> MQNSQDFSITELSLPKGGGAITGMGEALTPTGPDGMAALSLPLPISAGRGYAPAFTLNYNSGAGNSPFGLGWDCNVMTIRRRTHFGVPHYDETDTFLGPEGEVLVVADQPRDESTLQGINLGATFTVTGYRSRLESHFSRLEYWQPKTTGKTDFWLIYSPDGQVHLLGKSPQARISNPSQTTQTAQWLLEASVSSRGEQIYYQYRAEDDTGCEADEITHHLQATAQRYLHIVYYGNRTASETLPGLDGSAPSQADWLFYLVFDYGERSNNLKTPPAFSTTGSWLCRQDRFSRYEYGFEIRTRRLCRQVLMYHHLQALDSKITEHNGPTLVSRLILNYDESAIASTLVFVRRVGHEQDGNVVTLPPLELAYQDFSPRHHAHWQPMDVLANFNAIQRWQLVDLKGEGLPGLLYQDKGAWWYRSAQRLGEIGSDAVTWEKMQPLSVIPSLQSNASLVDINGDGQLDWVITGPGLRGYHSQRPDGSWTRFTPLNALPVEYTHPRAQLADLMGAGLSDLVLIGPKSVRLYANTRDGFAKGKDVVQSGEITLPVPGADPRKLVAFSDVLGSGQAHLVEVSATKVTCWPNLGRGRFGQPITLPGFSQPATEFNPAQVYLADLDGSGPTDLIYVHTNRLDIFLNKSGNGFAEPVTLRFPEGLRFDHTCQLQMADVQGLGVASLILSVPHMSPHHWRCDLTNMKPWLLNEMNNNMGVHHTLRYRSSSQFWLDEKAAALTTGQTPVCYLPFPIHTLWQTETEDEISGNKLVTTLRYARGAWDGREREFRGFGYVEQTDSHQLAQGNAPERTPPALTKNWYATGLPVIDNALSTEYWRDDQAFAGFSPRFTTWQDNKDVPLTPEDDNSRYWFNRALKGQLLRSELYGLDDSTNKHVPYTVTEFRSQVRRLQHTDSRYPVLWSSVVESRNYHYERIASDPQCSQNITLSSDRFGQPLKQLSVQYPRRQQPAINLYPDTLPDKLLANSYDDQQRQLRLTYQQSSWHHLTNNTVRVLGLPDSTRSDIFTYGAENVPAGGLNLELLSDKNSLIADDKPREYLGQQKTAYTDGQNTTPLQTPTRQALIAFTETTVFNQSTLSAFNGSIPSDKLSTTLEQAGYQQTNYLFPRTGEDKVWVAHHGYTDYGTAAQFWRPQKQSNTQLTGKITLIWDANYCVVVQTRDAAGLTTSAKYDWRFLTPVQLTDINDNQHLITLDALGRPITLRFWGTENGKMTGYSSPEKASFSPPSDVNAAIELKKPLPVAQCQVYAPESWMPVLSQKTFNRLAEQDWQKLYNARIITEDGRICTLAYRRWVQSQKAIPQLISLLNNGPRLPPHSLTLTTDRYDHDPEQQIRQQVVFSDGFGRLLQAAARHEAGMARQRNEDGSLIINVQHTENRWAVTGRTEYDNKGQPIRTYQPYFLNDWRYVSNDSARQEKEAYADTHVYDPIGREIKVITAKGWFRRTLFTPWFTVNEDENDTAAEVKKVKMPGSRPMKNIDPKLYQKTPTVSVYDNRGLIIRNIDFHRTTANGDPDTRITRHQYDIHGHLNQSIDPRLYEAKQTNNTIKPNFLWQYDLTGNPLCTESIDAGRTVTLNDIEGRPLLTVTATGVIQTRQYETSSLPGRLLSVAEQTPEEKTSRITERLIWAGNTEAEKDHNLAGQCVRHYDTAGVTRLESLSLTGTVLSQSSQLLIDTQEANWTGDNETVWQNMLADDIYTTLSTFDATGALLTQTDAKGNIQRLAYDVAGQLNGSWLTLKGQTEQVIIKSLTYSAAGQKLREEHGNDVITEYSYEPETQRLIGIKTRRPSDTKVLQDLRYEYDPVGNVISIRNDAEATRFWHNQKVMPENTYTYDSLYQLISATGREMANIGQQSHQFPSPALPSDNNTYTNYTRTYTYDRGGNLTKIQHSSPATQNNYTTNITVSNRSNRAVLSTLTEDPAQVDALFDAGGHQNTLISGQNLNWNTRGELQQVTLVKRDKGANDDREWYRYSGDGRRMLKINEQQASNNAQTQRVTYLPNLELRLTQNSTATTEDLQVITVGEAGRAQVRVLHWESGKPEDIDNNQLRYSYDNLIGSSQLELDSEGQIISEEEYYPYGGTALWAARNQTEASYKTIRYSGKERDATGLYYYGYRYYQPWIGRWLSSAPAGTIDGLNLYRMVRNNPVTLLDPDGLMPTIAERIAALKKNKVTDSAPSPANATNVAINIRPPVAPKPSLPKASTSSQPTTHPIGAANIKPTTSG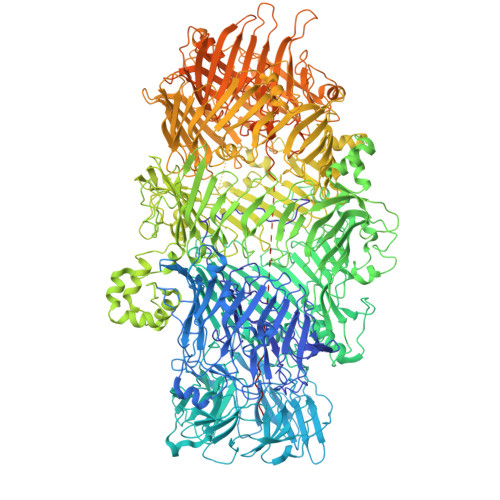SSIVAPLSPVGNKSTSEISLPESAQSSSSSTTSTNLQKKSFTLYRADNRSFEEMQSKFPEGFKAWTPLDTKMARQFASIFIGQKDTSNLPKETVKNISTWGAKPKLKDLSNYIKYTKDKSTVWVSTAINTEAGGQSSGAPLHKIDMDLYEFAIDGQKLNPLPEGRTKNMVPSLLLDTPQIETSSIIALNHGPVNDAEISFLTTIPLKNVKPHKR>AMAISNWVNVISDLKKIEDLIQSMHIDATLYTESDVHPSCKVTAMKCFLLELQVISLESGDASIHDTVENLIILANNSLSSNGNVTESGCKECEELEEKNIKEFLQSFVHIVQMFINTS[2x];>[2x]AMAISITCPPPMSVEHADIWVKSYSLYSRERYICNS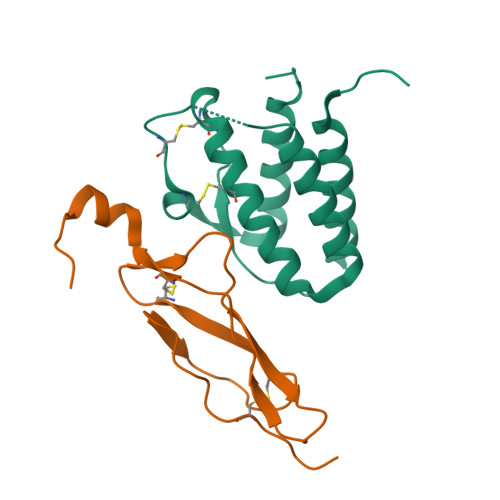GFKRKAGTSSLTECVLNKATNVAHWTTPSLKCIRDPALVHQRPAPPSTVTTAGVTPQPESLSPSGKEPAAS>MSSMNPEYDYLFKLLLIGDSGVGKSCLLLRFADDTYTESYISTIGVDFKIRTIELDGKTIKLQIWDTAGQERFRDITSSYYRGAHGIIVVYDVTDQESFNNVKQWLQEIDRYASENVNKLLVG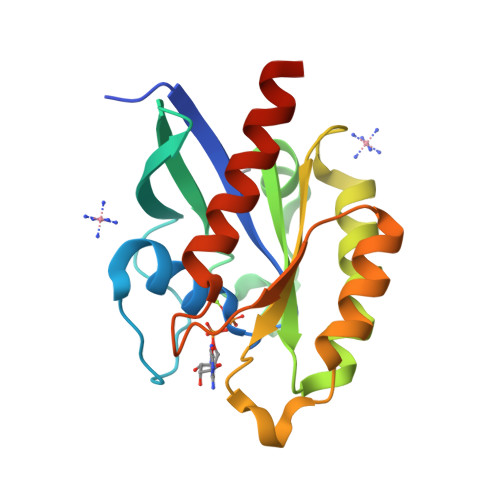NKCDLTTKKVVDYTTAKEFADSLGIPFLETSAKNATNVEQSFMTMAAEIKKRMLEHHHHHH[2x]> VVGGEDAKPGQFP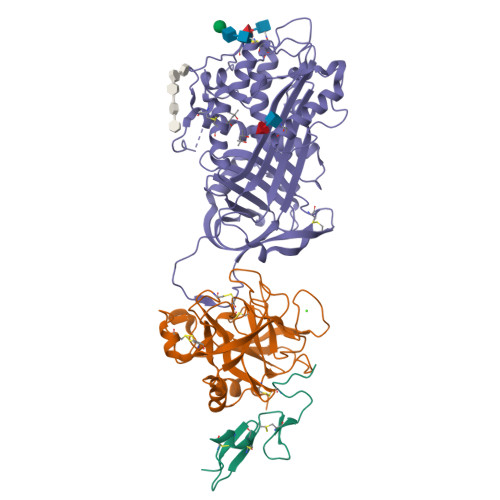WQVVLNGKVDAFCGGSIVNEKWIVTAAHCVETGVKITVVAGEHNIEETEHTEQKRNVIRIIPHHNYNAAINKYNHDIALLELDEPLVLNSYVTPICIADKEYTNIFLKFGSGYVSGWGRVFHKGRSALVLQYLRVPLVDRATCLRSTKFTIYNNMFCAGFHEGGRDSCQGDAGGPHVTEVEGTSFLTGIISWGEECAMKGKYGIYTKVSRYVNWIKEKTKLT;> HGSPVDICTAKPRDIPMNPMCIYRSPEKKATEDEGSEQKIPEATNRRVWELSKANSRFATTFYQHLADSKNDNDNIFLSPLSISTAFAMTKLGACNDTLQQLMEVFKFDTISEKTSDQIHFFFAKLNCRLYRKANKASKLVSANRLFGDKSLTFNETYQDISELVYGAKLQPLDFKENAEQSRAAINKWVSNKTEGRITDVIPSEAINELTVLVLVNTIYFKGLWKSKFSPENTRKELFYKADGESCSASMMYQEGKFRYRRVAEGTQVLELPFKGDDITMVLILPKPEKSLAKVEKELTPEVLQEWLDELEEMMLVVHMPRFRIEDGFSLKEQLQDMGLVDLFSPEKSKLPGIVAEGRDDLYVSDAFHKAFLEVNEEGSEAAASTAVVIAGRSLNPNRVTFKANRPFLVFIREVPLNTIIFMGRVANPCVK;> MDVTCNIKNGRCEQFCKNSADNKVVCSCTEGYRLAENQKSCEPAVPFPCGRVSVSQTSK>[4x]STAGKVIKCKAAVLWEEKKPFSIEEVEVAPPKAHEVRIKMVATGICRSDDHVVSGTLVTPLPVIAGHEAAGIVESIGEGVTTVRPGDKVIPLFTPQCGKCR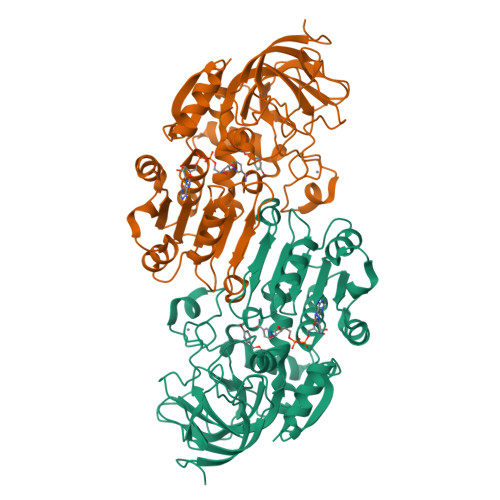VCKHPEGNFCLKNDLSMPRGTMQDGTSRFTCRGKPIHHFLGTSTFSQYTVVDEISVAKIDAASPLEKVCLIGCGFSTGYGSAVKVAKVTQGSTCAVFGLGGVGLSVIMGCKAAGAARIIGVDINKDKFAKAKEVGATECVNPQDYKKPIQEVLTEMSNGGVDFSFEVIGRLDTMVTALSCCQEAYGVSVIVGVPPDSQNLSMNPMLLLSGRTWKGAIFGGFKSKDSVPKLVADFMAKKFALDPLITHVLPFEKINEGFDLLRSGESIRTILTF>[2x]AL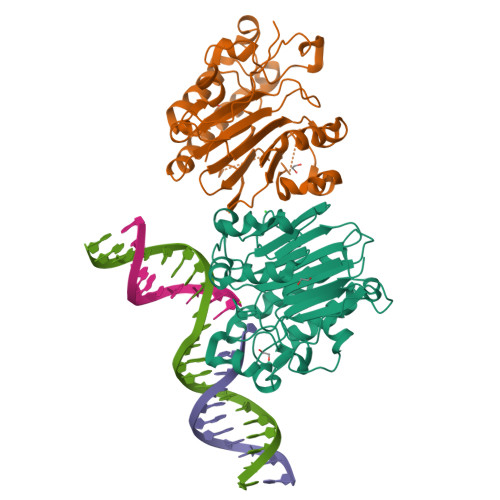YEDPPDQKTSPSGKPATLKICSWNVDGLRAWIKKKGLDWVKEEAPDILCLQETACSENKLPAELQELPGLSHQYWSAPSDKEGYSGVGLLSRQCPLKVSYGIGDEEHDQEGRVIVAEFDSFVLVTAYVPNAGRGLVRLEYRQRWDEAFRKFLKGLASRKPLVLCGDLNVAHEEIDLRNPKGNKKNAGFTPQERQGFGELLQAVPLADSFRHLYPNTPYAYTFWTYMMNARSKNVGWRLDYFLLSHSLLPALCDSKIRSKALGSDHCPITLYLAL> MAHHHHHHMSMRLIWAQSTSGIIGRDNSIPWRLPEDLARFKEMTMGHPVVMGRLTWESLPASVRPLPGRRNIVVTRDADYRA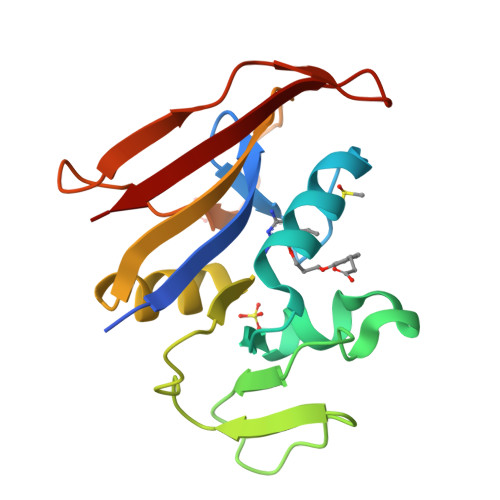EGAEVVTDLPDEPDAWVIGGAQIYAMALARADRCEVTEVDIALTPLDGDARAPVLDDSWVATTGEWQTSTSGLRFRFCSYRR> GHMAKTYDYLFKLLLIGDSGVGKTCVLFRFSEDAFNSTFISTIGIDFKIRTIELDGKRIKLQIWDTAGQERFRTITTAYYRGAMGIMLVYDITNEKSFDNIRNWIRNIEEHASADVEKMILGNKCD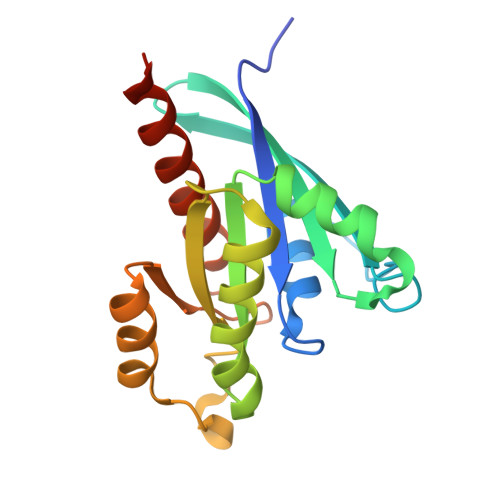VNDKRQVSKERGEKLALDYGIKFMETSAKANINVENAFFTLARDIKAKMDKKLEGNSPQG> GLKQKIVIKVAMEGNNCRSKAMALVASTGGVDSVALVGDLRDKIEVVGYGIDPIKLISALRKKVGDA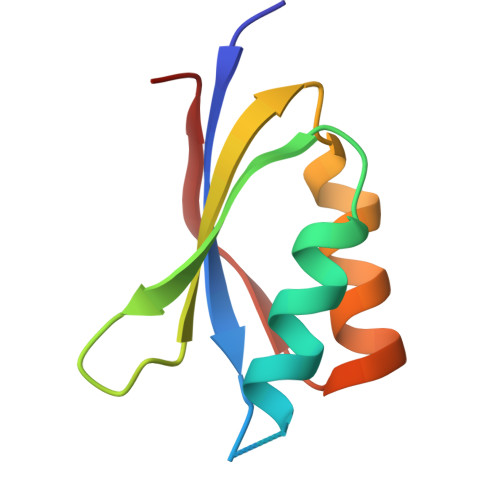ELLQVSQA> SAECPVVNELERINCIPDQPPTKATCDQRGCCWNPQGAVSVPWCYYSKNHSYHVEGNLVNTNAGFTARLKNLPSSPVFGSNVDNVLLTAEYQTSNRFHFKLTDQTNNRFEVPHEHVQSFSGNAAASLTYQVEISRQPFSIKVTRRSNNRVLFDSSIGPLLFADQFLQLSTRLPSTNVYGLGEHVHQQYRHDMNWKTWPIFNRDTTPNGNGTNLYGAQTFFLCLEDASGLSFGVFLMNSNAMEVVLQPAPAITYRTIGGILDFYVFLGNTPEQVVQEYLELIGRPALPSYWALGFHLSRYEYGTLDNMREVVERNRAAQLPYDVQHADIDYMDERRDFTYDSVDFKGFPEFVNELHNNGQKLVIIVDPAISNNSSSSKPYGPYDRGSDMKIWVNSSDGVTPLIGEVWPGQTVFPDYTNPNCAVWWTKEFELFHNQVEFDGIWIDMNEVSNFVDGSVSGCSTNNLNNPPFTPRILDGYLFCKTLCMDAVQHWGKQYDIHNLYGYSMAVATAEAAKTVFPNKRSFILTRSTFAGSGKFAAHWLGDNTATWDDLRWSIPGVLEFNLFGIPMVGP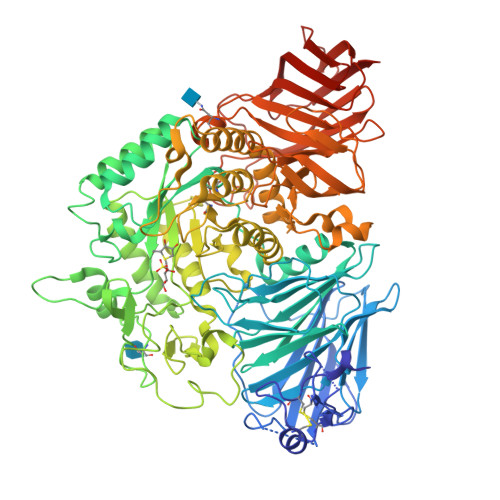DICGFALDTPEELCRRWMQLGAFYPFSRNHNGQGYKDQDPASFGADSLLLNSSRHYLNIRYTLLPYLYTLFFRAHSRGDTVARPLLHEFYEDNSTWDVHQQFLWGPGLLITPVLDEGAEKVMAYVPDAVWYDYETGSQVRWRKQKVEMELPGDKIGLHLRGGYIFPTQQPNTTTLASRKNPLGLIIALDENKEAKGELFWDDGETKDTVANKVYLLCEFSVTQNRLEVNISQSTYKDPNNLAFNEIKILGTEEPSNVTVKHNGVPSQTSPTVTYDSNLKVAIITDIDLLLGEAYTVEWAHHHHHH> YNVKPRQPEYKCIDSNLQYDCVFYDVHIDMQTQDVYFGFEDITLNNQKIVTFKNSTMRKLPAALLDSFRQVELLNLND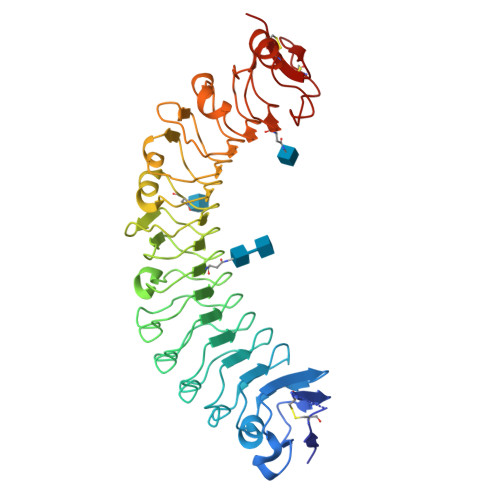LQIEEIDTYAFAYAHTIQKLYMGFNAIRYLPPHVFQNVPLLTVLVLERNDLSSLPRGIFHNTPKLTTLSMSNNNLERIEDDTFQATTSLQNLQLSSNRLTHVDLSLIPSLFHANVSYNLLSTLAIPIAVEELDASHNSINVVRGPVNVELTILKLQHNNLTDTAWLLNYPGLVEVDLSYNELEKIMYHPFVKMQRLERLYISNNRLVALNLYGQPIPTLKVLDLSHNHLLHVERNQPQFDRLENLYLDHNSIVTLKLSTHHTLKNLTLSHNDWDCNSLRALFRNVARPAVDDADQHCKIDYQLEHGLCCKES(2S)-2-[[(3S,4S)-5-cyclohexyl-4-[[(4S,5S)-5-[(2-methylpropan-2-yl)oxycarbonylamino]-4-oxidanyl-6-phenyl-hexanoyl]amino]-3-oxidanyl-pentanoyl]amino]-4-methyl-pentanoic acid | C34 H55 N3 O8 | 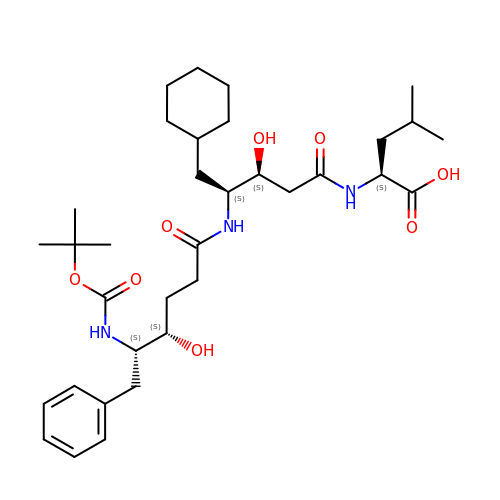UYUPAZNZXXOTIF-ZIUUJSQJSA-N>[2x]MKDRKILNE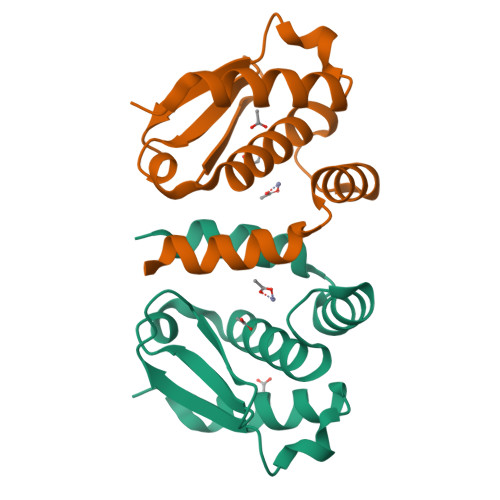ILSNTINELNLNDKKANIKIKIKPLKRKIASISLTNKTIYINKNILPYLSDEEIRFILAHELLHLKYGKYHINEFEEELLFLFPNKEAILFNLINKLFQKK> MTAASIDRELVPWSDPEFRNNPYPWYRRLQQDHPVHKLEDGTYLVSRYADVSHFAKLPIMSVEPGWADAGPWAVASDTALGSDPPHHTVLRRQTNKWFTPKLVDGWVRTTRELVGDLLDGVEAGQVIEARRDLAVVPTHVTMARVLQLPEDDADAVMEAMFEAMLMQSAEPADGDVDRAAVAFGYLSARVAEMLEDKRVNPGDGLADSLLDAARAGEITESEAIATILVFYAVGHMAIGYLIASGIELFA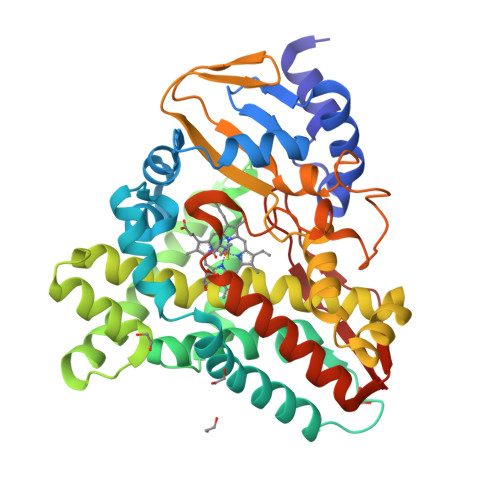RRPEVFTAFRNDESARAAIINEMVRMDPPQLSFLRFPTEDVEIGGVLIEAGSPIRFMIGAANRDPEVFDDPDVFDHTRPPAASRNLSFGLGPHSCAGQIISRAEATTVFAVLAERYERIELAEEPTVAHNDFARRYRKLPIVLS> GNAS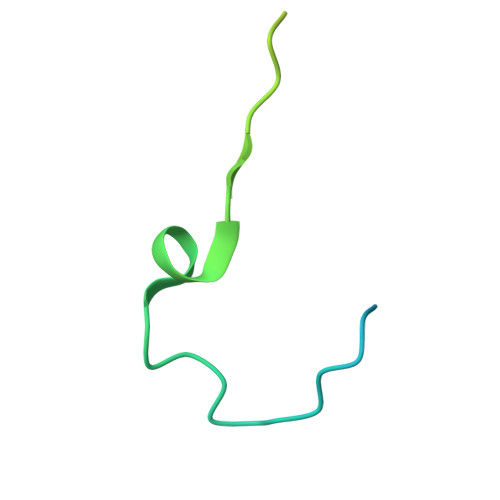SSDKSNSQSSGNEGVIINNFYSNQYQNSIDLSASGGNAGDAPQNNGQLSNILGGAANAFATMAPLLL>[6x]MTNSVSRDFSIERIIEAEQRAETQCGDRALTFLRVGPYSTVQPDYKGAVSALCQVVNKQLFQMVEYARMMPHFAQVPLDDQVILLKAAWIELLIANVAWCSIVSLDDGGAGGGGGGLGHDG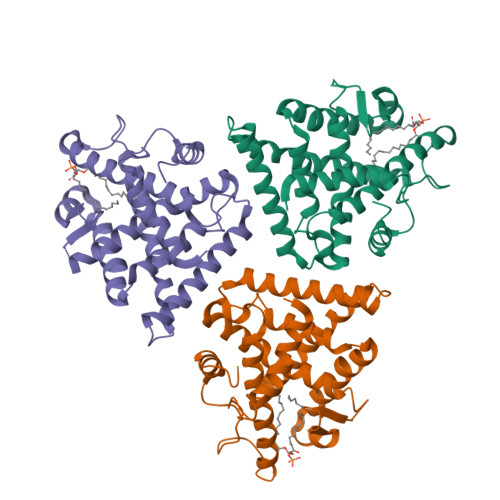SFERRSPGLQPQQLFLNQSFSYHRNSAIKAGVSAIFDRILSELSVKMKRLNLDRRELSCLKAIILYNPDIRGIKSRAEIEMCREKVYACLDEHCRLEHPGDDGRFAQLLLRLPALRSISLKCQDHLFLFRITSDRPLEELFLEQLEAPPPPGLAMKLE> AEVTQLSNGIVVATEHNPSAHTASVGVVFGSGAANENPYNNGVSNLWKNIFLSKENSAVAAKEGLALSSNISRDFQSYIVSSLPGSTDKSLDFLNQSFIQQKANLLSSSNFEATKKSVLKQVQDFEENDHPNRVLEHLHSTAFQNTPLSLPTRGTLESLENLVVADLESFANNHFLNSNAVVVGTGNIKHEDLVNSIESKNLSLQTGTKPVLKKKAAFLGSEVRLRDDTLPKAWISLAVEGEPVNSPNYFVAKLAAQIFGSYNAFEPASRLQGIKLLDNIQEYQLCDNFNHFSLSYKDSGLWGFSTATRNVTMIDDL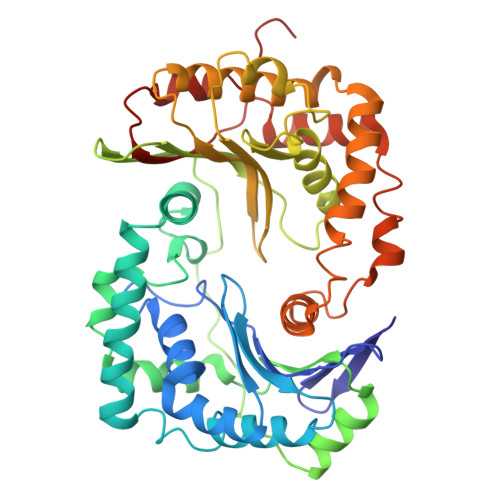IHFTLKQWNRLTISVTDTEVERAKSLLKLQLGQLYESGNPVNDANLLGAEVLIKGSKLSLGEAFKKIDAITVKDVKAWAGKRLWDQDIAIAGTGQIEGLLDYMRIRSDMSMMRW> TGRPEWIWLALGTALMGLGTLYFLVKGMGVSDPDAKKFYAITTLVPAIAFTMYLSMLLGYGLTMVPFGGEQNPIYWARYADWLFTTPLLLLDLALLVDADQG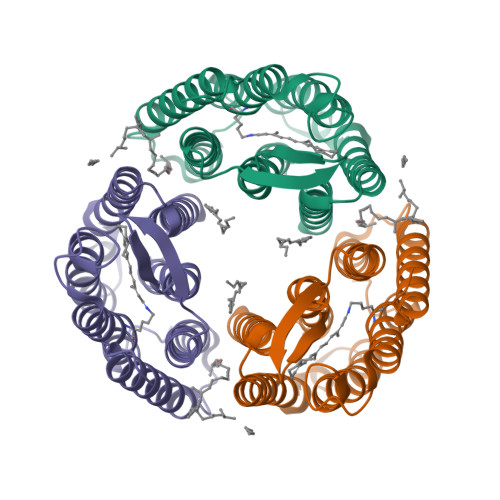TILALVGADGIMIGTGLVGALTKVYSYRFVWWAISTAAMLYILYVLFFGFTSKAESMRPEVASTFKVLRNVTVVLWSAYPVVWLIGSEGAGIVPLNIETLLFMVLDVSAKVGFGLILLRSRAIFG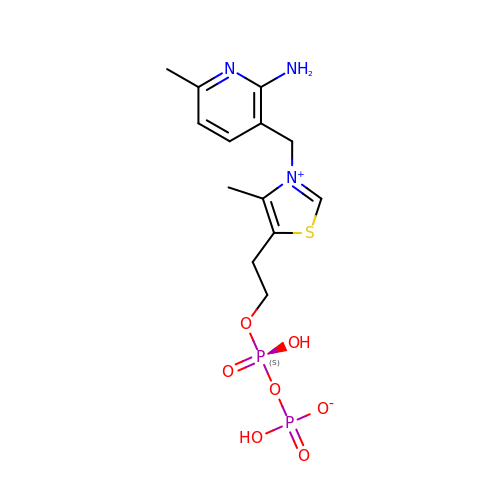1'-DEAZO-THIAMIN DIPHOSPHATE | C13 H19 N3 O7 P2 S | JHNXLHRDUXBCJW-UHFFFAOYSA-N>MPEQYRYTLPVKAGEQRLLGELTGAACATLVAEIAERHAGPVVLIAPDMQNALRLHDEISQFTDQMVMNLADWETLPYDSFSPHQDIISSRLSTLYQLPTMQRGVLIVPVNTLMQRVCPHSFLHGHALVMKKGQRLSRDALRTQLDSAGYRHVDQVMEHGEYATRGALLDLFPMGSELPYRLDFFDDEIDSLRVFDVDSQRTLEEVEAINLLPAHEFPTDKAAIELFRSQWRDTFEVKRDPEHIYQQVSKGTLPAGIEYWQPLFFSEPLPPLFSYFPANTLLVNTGDLETSAERFQADTLARFEN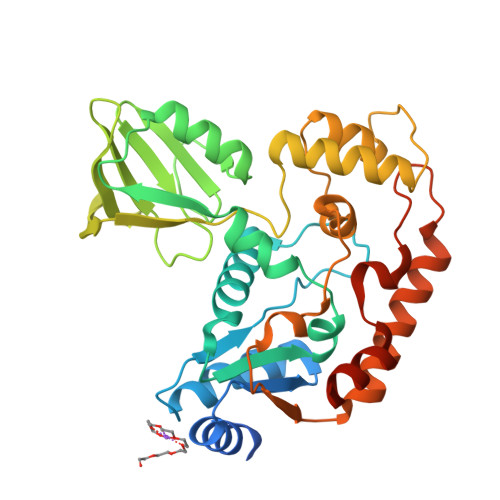RGVDPMRPLLPPQSLWLRVDELFSELKNAAALEHHHHHH[2x]>MIGKNIKSLRKTHDLTQLEFARIVGISRNSLSRYENGTSSVSTELIDIICQKFNVSYVDIVGEDKMLNPVEDYELTLKIEIVKERGANLLSRLYRYQDSQGISIDDESNPWILMSDDLSDLIHTNIYLVETFDEIERYSGYLDGIERMLEISEKRMVA[4x];>[4x]MEIQDYTDSEFKHALARNLRSLTRGKKSSKQPIAILLGGQSGAGKTTIHRIKQKEFQGNIVIIDGDSFRSQHPHYLELQQEYGKDSVEYTKDFAGKMVESLVTKLSSLGYNLLIEGTLRTVDVPKKTAQLLKNKGYEVQLALIATKPELSYL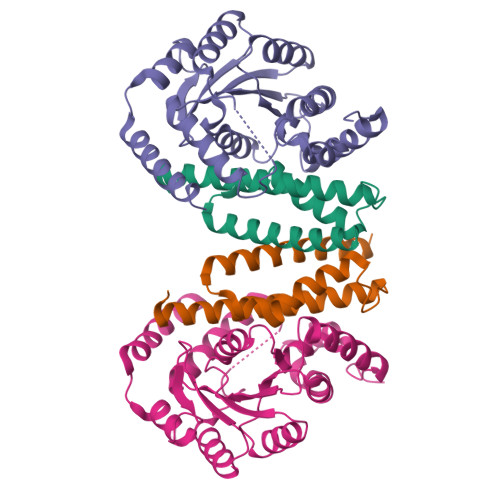STLIRYEELYIINPNQARATPKEHHDFIVNHLVDNTRKLEELAIFERIQIYQRDRSCVYDSKENTTSAADVLQELFFGEWSQVEKEMLQVGEKRLNELLEK Here, using a combination of bioinformatic, biochemical, and genetic analyses, we discovered and functionally characterized an unreported flavone reductase (FLR) that specifically catalyzes the hydrogenation reaction towards flavones and flavonols, and initiates their metabolism in F. plautii ATCC 49531 as a key step. The underlying molecular mechanism was intensively elucidated by analyzing the crystal structure of FLR as well as the co-crystal structures of FLR and its substrates. Of note, FLR and its widespread homologs represent an unreported class of ene-reductases with highly distinct amino acid sequence and catalytic property compared with those of all known ene-reductases. FLR-like enzymes were abundant in the human gut microbiota as well as other microbes living within flavonoid-rich environments, thereby suggesting a broad role of these ene-reductases in microbial communities.

To further illuminate the underlying mechanism, we solved the complex structures of FLR with various substrates, including apigenin, chrysin, and luteolin that contain similar A/C rings but differ in the B ring. The structures were refined to 2.55, 2.65, and 2.25 Å resolution, respectively, which adopt a very similar conformation with r.m.s.d. value of 0.18~0.21 Å. The substrate and the cofactor FMN bind in the same pocket, which is located at the dimer structure interface and mainly comprised of the N-terminal domain from one molecule and the C-terminal subdomain-2 from the neighbor molecule. The structures clearly demonstrate that the coordination of substrate mainly involves the A/C rings, while the B ring protrudes out of the pocket. Specifically, the A/C rings of substrates stack against the isoalloxazine ring of FMN on one side and the side chain of residue Ile275 of subdomain-2 on the other side. This substrate-binding pattern may explain why FLR can catalyze the reaction of apigenin, chrysin, and luteolin, since all these three substrates differ only in the B ring.

> MKILGISGGMRNGSNDGMCIEALMGAKEMGAEVEFIQLQNLHIEHCTGCTACVQSVLGGRGGKCVLKDDFDWLLDKMLDADGIVFSTPIFEKGATGLFHTITDRFGPRMDRGNNIIGTKIAEETGGTAPDPRILKDKVISFMSVGGSDWVTRTQCDAGMLALTPMWKVIDNEVFPWALSILVEDERVARAHQIGRNIAEAAKDIEHAQYQGDAGVCPHCHSRNFHLQDGKAICCLCGLEGEIHNEGGKYSFTFPAEQLEHAHDTLSGKFIHGNDIKENTGKKIANMQTEKYKARQAAYRAFITATVPEKG>MSIKFELIDVPIPQGTNVIIGQAHFIKTVEDLYEALVTSVPGVKFGIAFCEASGKRLVRHEANDEELRNLAIDLCKKIAAGHVFVIYIRNAWPINVLNAIKNVPEVVRIFAATANPLKVIVAEVEPERRGV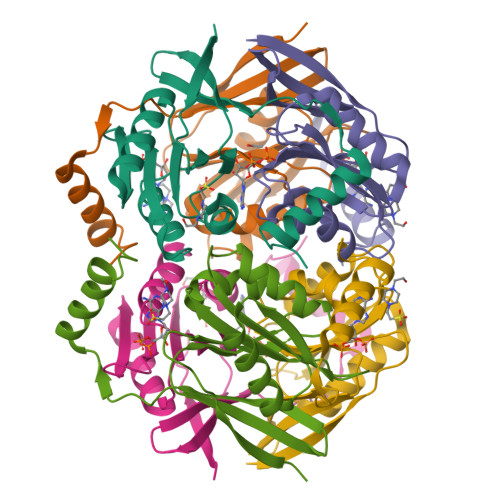VGVVDGHSPLGVETEKDREERKKFLREVVKYKL[3x]> FE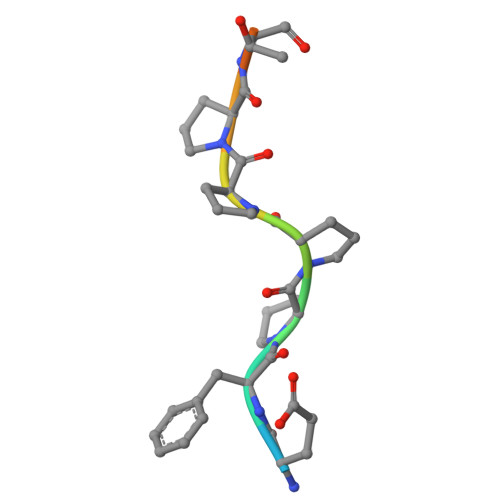FPPPPTDEE> ANEVNVYSYRQPYLIEPMLKNFEKDTGIKVNIIFADKGLVDRVKQEGELSPADVLLTVDISRVMEIVNADLAQKIDSKVLEKNIPAQFRDSNDQWFGLTTRARVIYTSKDRVGKLPAGFDYLDLAKPEYKGKVCVRSGKNSYNVSLFAAMIEHYGIEKTKAFLEGLKANLARKPQGGDRDQVKAIKEGICDYSIGNSYYYGKMLDDEKQKSWAEAAIINFPSGEHGTHKNISGVVIAKHSPNKANAVKLIEYLSGEKAQGLYAELNHEYPVKEGIEPSAIV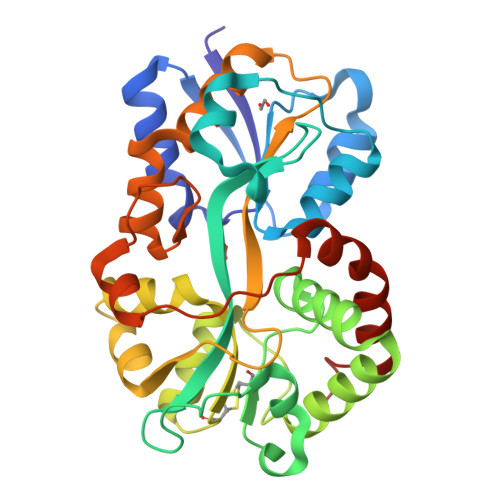KGWGTFKSDTIKLEDIAKNYEAALKLVDEVKFDDFSEKK>MAAAVRSVKGLVAVITGGASGLGLSTAKRLVGQGATAVLLDVPNSEGETEAKKLGGNCIFAPANVTSEKEVQAALTLAKEKFGRIDVAVNCAGIAVAIKTYHEKKNQVHTLEDFQRVINVNLIGTFNVIRLVAGVMGQNEPDQGGQRGVIINTASVAAFEGQVGQAAYSASKGGIVGMTLPIARDLAPIGIRVVTIAPGLFATPLLTTLPDKVRNFLASQVPFPSRLGDPAEYAHLVQMVIENPFLNGEVIRLD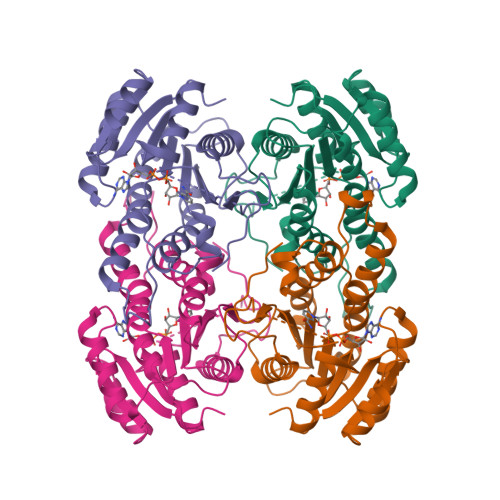GAIRMQP[4x]> METKRVNGTDRPPISSWSVDDVSNFIRELPGCQDYVDDFIQQEIDGQALLRLKEKHLVNAMG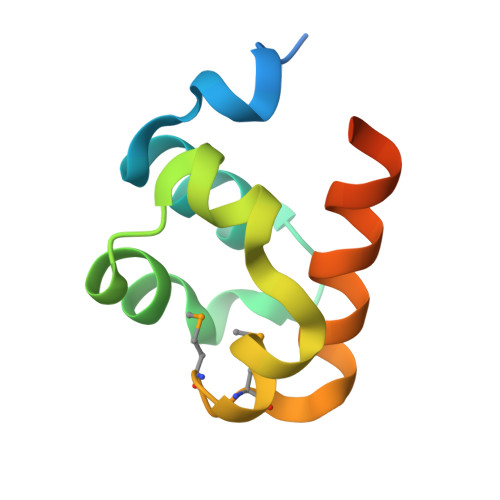MKLGPALKIVAKVESIKEVRDHHHHHH The voltage-gated potassium channel AKT1 is responsible for primary K+ uptake in Arabidopsis roots. AKT1 is functionally activated through phosphorylation and negatively regulated by a potassium channel α-subunit AtKC1. AKT1 is the first characterized hyperpolarization-activated voltage-dependent K+ channel in Arabidopsis thaliana, which belongs to the Shaker K+ channel family. Each subunit can be divided into four parts: the transmembrane segments comprising S1–S6 and the pore loop; the C-linker which contains the helices A’B’C’D’; and the CNBD.

In total, 181,714 particles were used for auto-refinement, yielding a final reconstruction of AKT1 map at an overall resolution of 3.4 Å. The model of 3D classification displayed a 2-fold but not 4-fold symmetric assembly at the cytoplasmic domain (CPD). Two pairs of diagonal subunits sharing the same conformation are named as Mol I/I’ and Mol II/II’. The pore domain of AKT1 displays a closed inner gate, with its narrowest constriction formed by I285. In Mol I/I’, the helices B’ and C’ of these two C-linkers are pushed into a relatively “straight” helix. By contrast, the helices B’ and C’ from C-linkers of Mol II and II’ exhibit a “kinked” conformation. In our study, loops1/1’ stack against “straight” C-linkers of AKT1 and might affect the downward movement of S4. The two “straight” C-linkers may sterically restrict the conformational change of the neighboring C-linkers, thus inhibiting the opening of the pore. These structural findings may underlie the low-activity of AKT1 in the basal state. In addition, four phospholipids are built surrounding the pore helices of AKT1.

>MASDYKDDDDKASDEVDAGTATMRGGALLCGQVQDEIEQLSRESSHFSLSTGILPSLGARSNRRVKLRRFVVSPYDHKYRIWEAFLVVLVVYTAWVSPFEFGFLRKPRPPLSITDNIVNAFFAIDIIMTFFVGYLDKSTYLIVDDRKQIAFKYLRSWFLLDLVSTIPSEAAMRISSQSYGLFNMLRLWRLRRVGALFARLEKDRNFNYFWVRCAKLVCVTLFAVHCAACFYYLIAARNSNPAKTWIGANVANFLEESLWMRYVTSMYWSITTLTTVGYGDLHPVNTKEMIFDIFYMLFNLGLTAYLIGNMTNLVVHGTSRTRNFRDTIQAASNFAHRNHLPPRLQDQMLAHLCLKYRTDSEGLQQQETLDALPKAIRSSISHFLFYSLMDKVYLFRGVSNDLLFQLVSEMKAEYFPPKEDVILQNEAPTDFYILVNGTADLVDVDTGTESIVREVKAGDIIGEIGVLCYRPQLFTVRTKRLCQLLRMNRTTFLNIIQANVGDGTIIMNNLLQHLKEMNDPVMTNVLLEIENMLARGKMDLPLNLCFAAIREDDLLLHQLLKRGLDPNESDNNGRTPLHIAASKGTLNCVLLLLEYHADPNCRDAEGSVPLWEAMVEGHEKVVKVLLEHGSTIDAGDVGHFACTAAEQGNLKLLKEIVLHGGDVTRPRATGTSALHTAVCEENIEMVKYLLEQGADVNKQDMHGWTPRDLAEQQGHEDIKALFREKLHERRVHIETSSSVPILKTGIRFLGRFTSEPNIRPASREVSFRIRETRARRKTNNFDNSLFGILANQSVPKNGLATVDEGRTGNPVRVTISCAEKDDIAGKLVLLPGSFKELLELGSNKFGIVATKVMNKDNNAEIDDVDVIRDGDHLIFATDS[4x]>[2x]HQRKVVSWIDVYTRATCQPREVVVPLTVELMGTVAKQLVPSCVTVQRCGGCCPDDGLECVPTGQHQVRMQILMIRYPSSQLGEMSLEEHSQCECRPK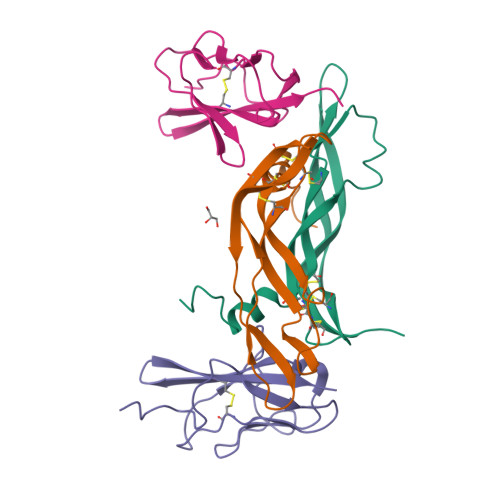KK;>[2x]SDTGRPFVEMYSEIPEIIHMTEGRELVIPCRVTSPNITVTLKKFPLDTLIPDGKRIIWDSRKGFIISNATYKEIGLLTCEATVNGHLYKTNYLTHRQT> SMNTDPLLPGFDYLTLHTSAARLRVAVKGSGPPLLLLHGYPQTHLAWHRIAPRLAEDYSVVLADLRGYGESRALDEEGADYSKAALARDQLETMGQ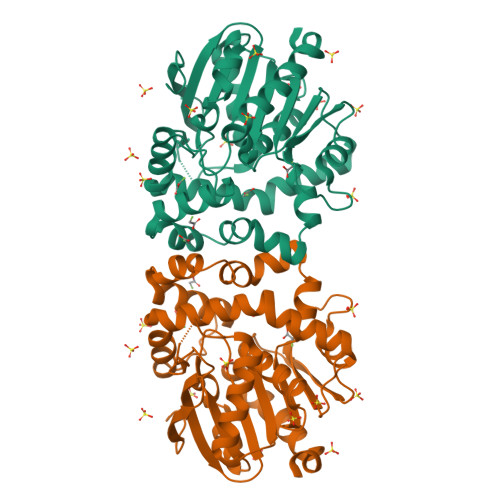LGFERFAVIGHDRGARVGYRLALDHPQAVAAFVSLTVVPILDNWAAVNKVFALNAYHWFLLAQPYDLPERLIGADPEHFLDYTLRRMAQGRDIYHPQALESYRRAFRDPAVRHAMCEDYRAAVGVDADADQADRDAGRRLQCPVQVLWEERPYAAGQHPLEIWKTWAGQVEGAAIGASHMLPEDAPDAVLEHLLGFLASHREALR> GQNAQAKMIAAQTAAGRRQAMEIMRQTNIQNADLSLQA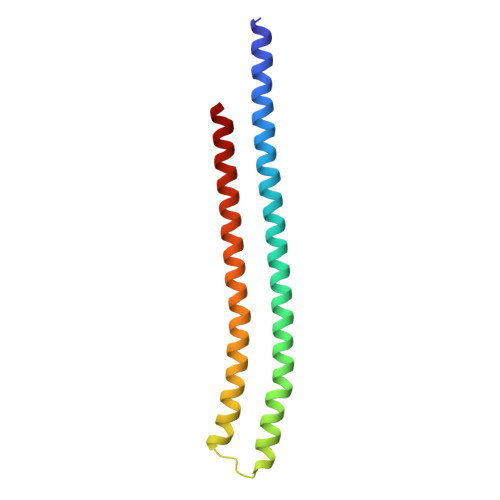RSKLEEASAELTSQNMQKVQAIGSIRAAIGESMLEGSSMDRIKRVTEGQFIREANMVTENYRRDYQAIFAQQLGGTQSAASQIDEIYKS> MKHHHHHHHGAAGTSLYKKAGENLYFQGSMAPRAGFDAEQVRDKARKDLLHLLEGVRGKKNLVIEKDLAGPLGVIVKASTLRDYGVDNFFFLENKNTGTSQRNIVFIARGESVRNAHAIAAQIKRIQRESQTSHDFHIFWVPRRTLFSDKVLEEAGVLGDANISELPLYFFPLERDVLSLELNDSFRDLYLAKDPTPVFLLSRALMGIQKKHGLFPRIIGKGENAKRVADLLSRMRQELLAGEEAGESDRAGLSPSTTIESVIIIDREVDFVTPLLTQLTYEGLIDEYFGIQNNQTDVDAVIVGAPAQSAASTSTAVPTNSSQSRKRKIQLDGSDSLYSQLRDANFAIVGSLLNTVARRLKSDYESRHNTKTTAELKEFVKKLPGYQAEQQSLKIHSNIAEEIINYTRTEIFNKLLEVQQNLAAGADPSSQFDSIEELVARDTPLPQVLRLLCLYSCISGGIKTKELDHFRRLVLQGYGHQHLLTLHNLERLQMFLSKSSPLASMITMSGSSGGPDQKTNYTYLRKQLRLIVDEVNEQDPNDIAYVYSGYAPLSIRLVQCVLQKQYLLSITKGSGTVIAAGPVAGGGAQGWKGFEEIVKHARGPTFDEIQKGEDKAVKARALLSGSSGDKKTVFVVFVGGITFTEIAALRFIAKQEEARRNIVICTTSIINGNRMMNAAIETATFEKTTVTTA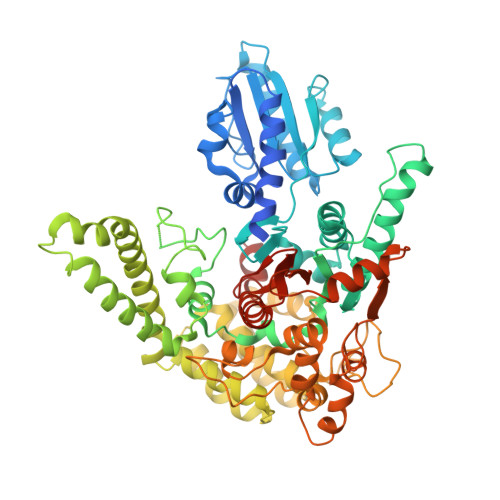AAQ> MGSDKIHHHHHHMKIAVLPGDGIGPEVVREALKVLEVVEKKTGKTFEKVFGHIGGDAIDRFGEPLPEETKKICLEAD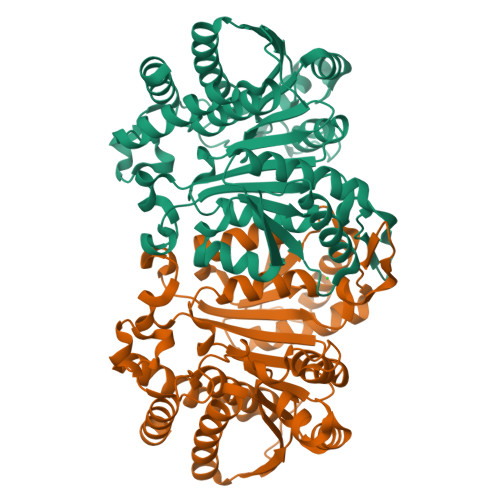AIFLGSVGGPKWDDLPPEKRPEIGGLLALRKMLNLYANIRPIKVYRSLVHVSPLKEKVIGSGVDLVTVRELSYGVYYGQPRGLDEEKGFDTMIYDRKTVERIARTAFEIAKNRRKKVTSVDKANVLYSSMLWRKVVNEVAREYPDVELTHIYVDNAAMQLILKPSQFDVILTTNMFGDILSDESAALPGSLGLLPSASFGDKNLYEPAGGSAPDIAGKNIANPIAQILSLAMMLEHSFGMVEEARKIERAVELVIEEGYRTRDIAEDPEKAVSTSQMGDLICKKLEEIW>[2x]ELEIEWHKFETSEEIISTYLIDDVLYTGVNGAVYTFSNNELNKTGLTNNNNYITTSIKVEDTLVCGTNNGNPKCWKIDGSEDPKYRGRGYAPYQNSKVTIISHNECVLSDINISKEGIKRWRRFDGPCGYDLYTADNVIPKDGVRGAFVDKDGTYDKVYILFTDTIDTKRIVKIPYIAQMCLNDEGGPSSLSSHRWSTFLKVELECDIDGRSYRQIIHSKAIKTDNDTILYVFFDSPYSKSALCTYSMNAIKHSFSTSKLGGYTKQLPSPAPGICLPAGKVVPHTTFDIIEQYNELDDIIKPLSQPIFEGPSGVKWFDIKEKENEHREYRIYFIKENTIYSFDTKSKQTRSAQVDARLFSVMVTSKPLFIADIGIGVGIPRMKKILKMGTHHHHHHHH;>ADEPVWRSEQAIGAIAASQEDGVFVASGSCLDQLDYSLEHSLSRLYRDQAGNCTEPVSLAPPARPRPGSSFSKLLLPYREGAAGLGGLLLTGWTFDRGACEVRPLGNLSRNSLRNGTEVVSCHPQGSTAGVVYRAGRNNRWYLAVAATYVLPEPETASRCNPAASDHDTAIALKDTEGRSLATQELGRLKLCEGAGSLHFVDAFLWNGSIYFPYYPYNYTSGAATGWPSMARIAQSTEVLFQGQASLDCGHGHPDGRRLLLSSSLVEALDVWAGVFSAAAGEGQERRSPTTTALCLFRMSEIQARAKRVSWDFKTAESHCKEGDQPERVQPIA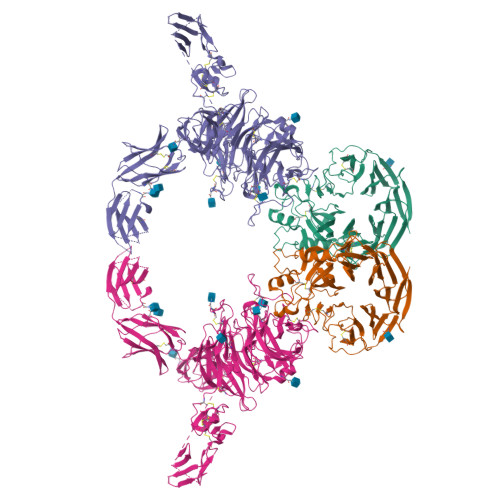SSTLIHSDLTSVYGTVVMNRTVLFLGTGDGQLLKVILGENLTSNCPEVIYEIKEETPVFYKLVPDPVKNIYIYLTAGKEVRRIRVANCNKHKSCSECLTATDPHCGWCHSLQRCTFQGDCVHSENLENWLDISSGAKKCPKIQIIRSSKEKTTVTMVGSFSPRHSKCMVKNVDSSRELCQNKSQPNRTCTCSIPTRATYKDVSVVNVMFSFGSWNLSDRFNFTNCSSLKECPACVETGCAWCKSARRCIHPFTACDPSDYERNQEQCPVAVEKTSGGGRPKENKGNRTNQALQVFYIKSIEPQKVSTLGKSNVIVTGANFTRASNITMILKGTSTCDKDVIQVSHVLNDTHMKFSLPSSRKEMKDVCIQFDGGNCSSVGSLSYIALPHCSLIFPATTWISGGQNITMMGRNFDVIDNLIISHELKGNINVSEYCVATYCGFLAPSLKSSKVRTNVTVKLRVQDTYLDCGTLQYREDPRFTGYRVESEVDTELEVKIQKENDNFNISKKDIEITLFHGENGQLNCSFENITRNQDLTTILCKIKGIKTASTIANSSKKVRVKLGNLELYVEQESVPSTWYFLIVLPVLLVIVIFAAVGVTRHKSKELSRKQSQQLELLESELRKEIRDGFAELQMDKLDVVDSFGTVPFLDYKHFALRTFFPESGGFTHIFTEDMHNRDANDKNESLTALDALICNKSFLVTVIHTLEKQKNFSVKDRCLFASFLTIALQTKLVYLTSILEVLTRDLMEQCSNMQPKLMLRRTESVVEKLLTNWMSVCLSGFLRETVGEPFYLLVTTLNQKINKGPVDVITCKALYTLNEDWLLWQVPEFSTVALNVVFEKIPENESADVCRNISVNVLDCDTIGQAKEKIFQAFLSKNGSPYGLQLNEIGLELQMGTRQKELLDIDSSSVILEDGITKLNTIGHYEISNGSTIKVFKKIANFTSDVEYSDDHCHLILPDSEAFQDVQGKRHRGKHKFKVKEMYLTKLLSTKVAIHSVLEKLFRSIWSLPNSRAPFAIKYFFDFLDAQAENKKITDPDVVHIWKTNSLPLRFWVNILKNPQFVFDIKKTPHIDGCLSVIAQAFMDAFSLTEQQLGKEAPTNKLLYAKDIPTYKEEVKSYYKAIRDLPPLSSSEMEEFLTQESKKHENEFNEEVALTEIYKYIVKYFDEILNKLERERGLEEAQKQLLHVKVLFDEKKKCKWMGTSSGLEVLFQ[2x]>ARDISIEDLLARKPKDLDDSAVAAFLKDKVVLVSGAGGTIGSELCKQCIKFGAKHLIMVDHSEYNLYKINDDLNLYKEKITPILLSILDKQSLDEVLKTYKPELILHAAAYKHVPLCEQNPHSAVINNILGTKILCDSAKENKVAKFVMISTDKAVRPTNIYGCTKRVCELYTLSMSDENFEVACVRFGNVLGSSGSVIP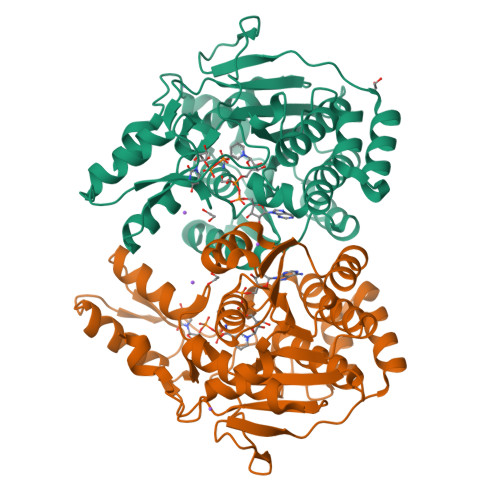KFKAQIANNEPLTLTHPDIVRYFMLVAEAVQLVLQAGAIAKGGELFVLDMGKPVKIIDLAKKMLLLSNRNDLEIKITGLRKGEKLYEELLIDENDAKTQYESIFVAKNEKVDLDWLNKEIENLQICEDISEALLKIVPEFKHNKEGIAAGFNRIPAAALEHHHHHH[2x]> MDKTFINCVSRSPTGFSPALVMDGISYNASSQQVYNRLVEFKRGSTDIEPALAESWTVSDDGLTYTFNLRKGVKFHSNKEFTPSRDFNADDVVFSFQRQLDPNHPYHNVSKATYPYFKAMKFSTLLKSVEKVDMHTVKITLNRQDATFLASLGMDFISIYSAEYADKMLAAGKPETIDTTPIGTGPFLFAGYQVDQKSRYLAHKEYWKGKADIDRLIFEIVPDATARYAKLQAGACDLIDFPNAADLEKMKTDPKVNLHSQSGLNIAYIAFNTEKAPFDNVKVRQALNYAVDKNAIIDAVYRGAGVAAKNPLPPTIWGYNNEITGYEYSPEKAKQLLKEAGFENGFETDIWVQPVVRASNPNPRRMAE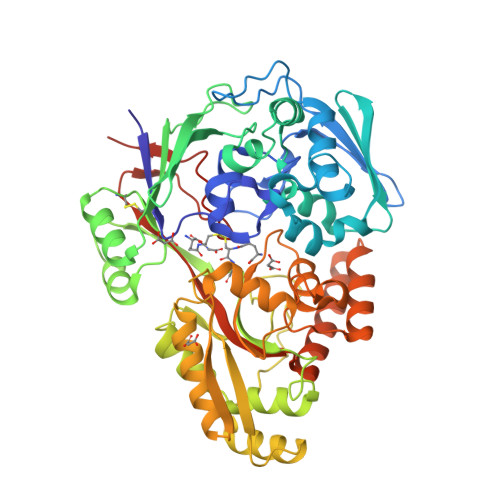LVQSDWEKVGVKSKLVSYEWGDYIKRTKAGELTAGTYGWSGDNGDPDNFLSPLFGSENVGNSNYARFKNPELDALLHKAVGLSDKAERAKIYEQAQVLLKEQAPWINVAHSINFAPTSKRVQDYKQSPFGYTYLYGTKLADKLAAALEHHHHHH> AFVVTDNCIKCKYTDCVEVCPVDCF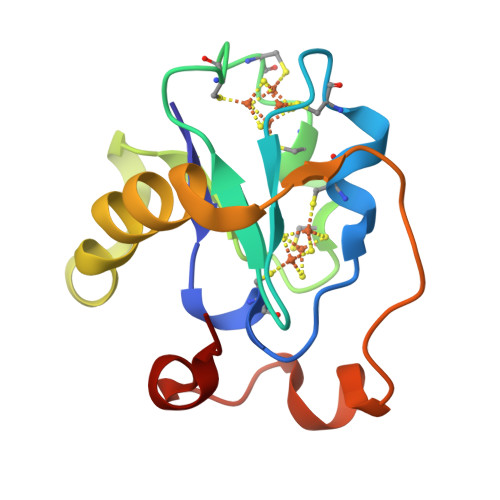YEGPNFLVIHPDECIDCALCAPECPAQAIFSEDEVPEDMQEFIQLNAELAEVWPNITEKKDPLPDAEDWDGVKGKLQHLER>GSHMNGLIYAVGGFATLETESGELVPTELNSVEAYDPERNEWSLVAPLSTRRSGVGVAVLNGLIYAVGGYDGSPD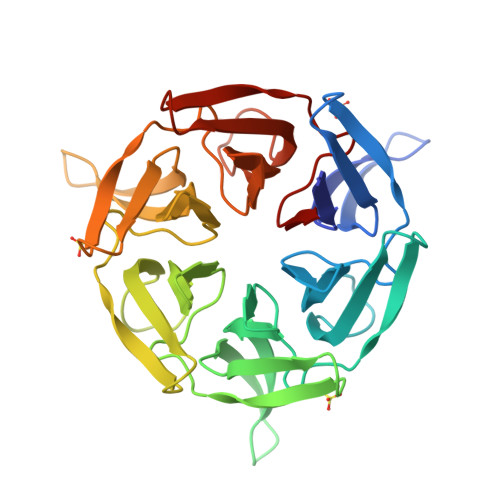GSTHLNSVEAYDPERNEWSLVAPLSTRRSGVGVAVLNGLIYAVGGFATLETESGELVPTELNSVEAYDPERNEWSLVAPLSTRRSGVGVAVLNGLIYAVGGYDGSPDGSTHLNSVEAYDPERNEWSLVAPLSTRRSGVGVAVLNGLIYAVGGFATLETESGELVPTELNSVEAYDPERNEWSLVAPLSTRRSGVGVAVLNGLIYAVGGYDGSPDGSTHLNSVEAYDPERNEWSLVAPLSTRRSGVGVAVL[2x]> MSEQSQLDD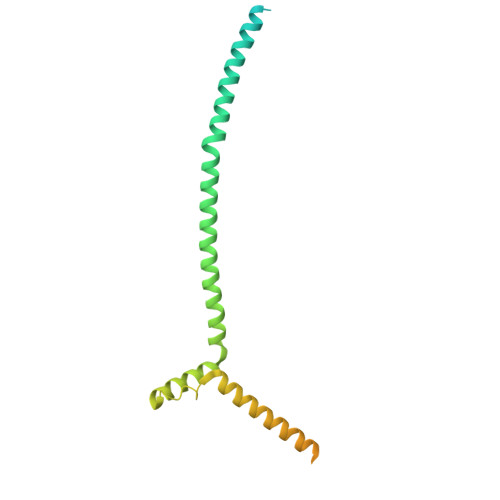STIDKLIPQIFNEMRSNLNNTTNKFPKSTGGGASDNISANSNSIRSFNSITTQSLLKESESLDKITAMIKNVTAALKNNLPVYVNQVHEVCKSTNSILDSWINIHSQAGYIHKLMSDQTYLKLINDRLHNENVNTNDEDGSTLHNVIALKKKEILDLRQKLENRKGEKDAAPAKPPNQGLNPRYGVQSGRRPVPSAGISNNGRVRKTHVPASKRPSGIPRVTNRWTKPTASSSRKMFR>[7x]MSDLDRLASRAAIQDLYSDQLIGVDKRQEGRLASIWWDDAEWTIEGIGTYKGPEGALDLA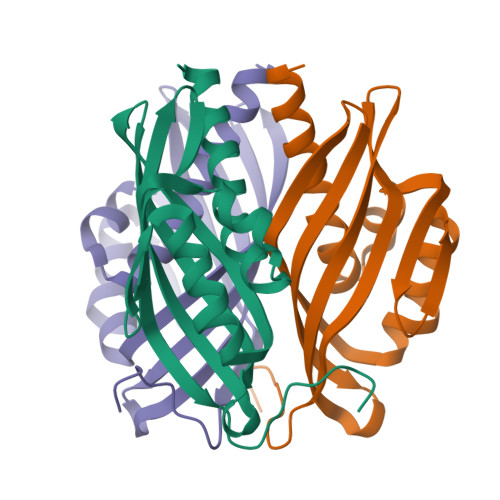NNVLWPMYHETIHYGTNLRLEFVSADKVNGIGDVLCLGNLVEGNQSILIAAVYTNEYERRDGVWKFSKLNGCMNYFTPLAGIHFAPPGIHFAPSGA>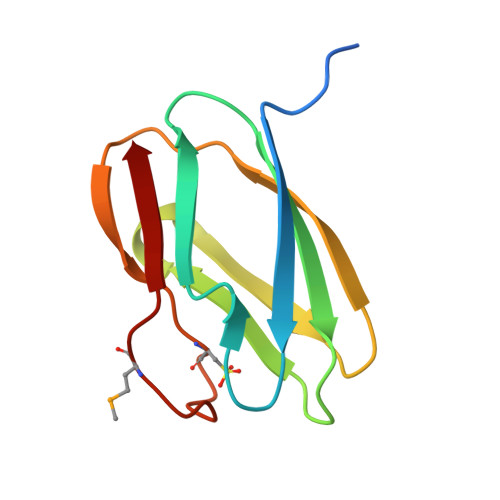SNANDLAQPIASAKVIEVELNDDYFNPNVITIPINESTTLLLKNKGKSEHTFTIKKLGIDVVVESGKEKNITVKPKSAGTYELICRYHLLKGMEGKVIVK[2x]>[3x]GSGIIKLRKEIERLEEKLEDANERIAELVKLEERQRIARDLHDTLGQKLSLIGLKSDLARKLIYKDPEQAARELKSVQQTARTSLNEVRKIVSSMKGIRLKDELINIKQILEAADIMFIYEEEKWPENISLLNENILSMCLKEAVTNVVKH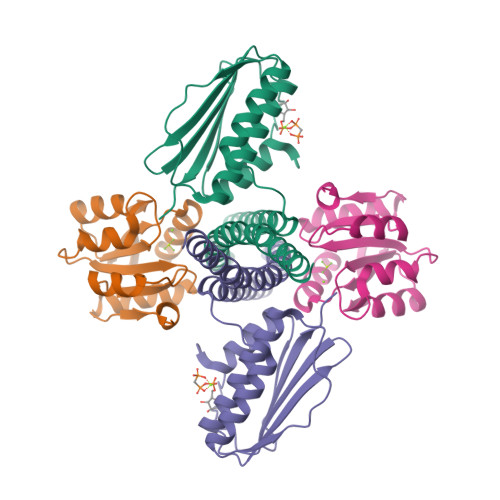SQAKTCRVDIQQLWKEVVITVSDDGTFKGEENSFSKGHGLLGMRERLEFANGSLHIDTENGTKLTMAIPNNSK;>[3x]GSGSMISIFIAEDQQMLLGALGSLLNLEDDMEVVGKGTTGQDAVDFVKKRQPDVCIMDIEMPGKTGLEAAEELKDTGCKIIILTTFARPGYFQRAIKAGVKGYLLKDSPSEELANAIRSVMNGKRIYAPELMEDLYSEA5'-azido-8-bromo-5'-deoxyadenosine | 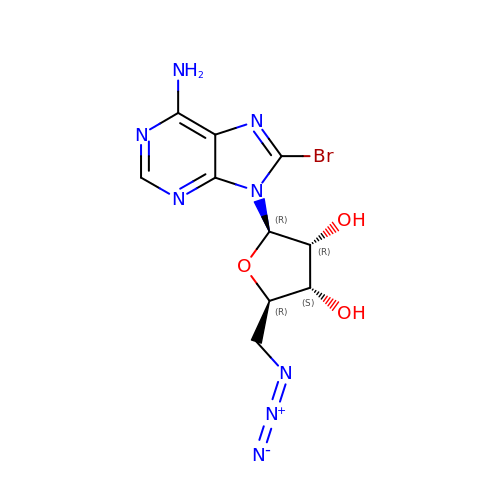C10 H11 Br N8 O3 | USVISQHKGJAQDS-UUOKFMHZSA-N> MSKPELKEDKMLEVHFVGDDDVLNHILDREGGAKLKKERAQLLVNPKKIIKKPEYDLEEDDQEVLKDQNYVEIMGRDVQESLKNGSATGGGNKVYSFQNRKHSEKMAKLASELAKTPQKSVSFSLKNDPEITINVPQSSKGHSASDKVQPKNNDKSEFLSTAPRSLRKRLIVPRSHSDSESEYSASNSEDDEGVAQEHEEDTNAVIFSQKIQAQNRVVSAPVGKETPSKRMKRDKTSDLVEEYFEAHSSSKVLTSDRTLQKLKRAKLDQQTLRNLLSKVSPSFSAELKQLNQQYEKLFHKWMLQLHLGFNIVLYGLGSKRDLLERFRTTMLQDSIHVVINGFFPGISVKSVLNSITEEVLDHMGTFRSILDQ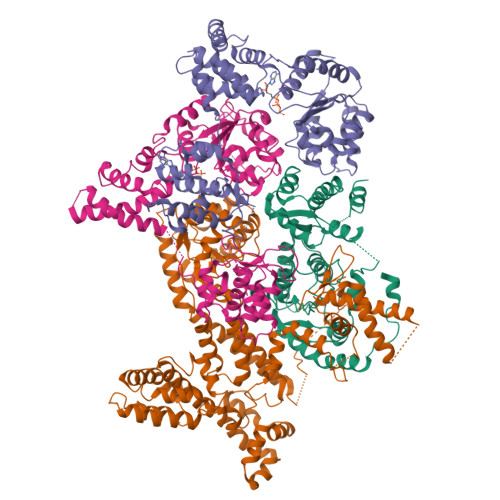LDWIVNKFKEDSSLELFLLIHNLDSQMLRGEKSQQIIGQLSSLHNIYLIASIDHLNAPLMWDHAKQSLFNWLWYETTTYSPYTEETSYENSLLVKQSGSLPLSSLTHVLRSLTPNARGIFRLLIKYQLDNQDNPSYIGLSFQDFYQQCREAFLVNSDLTLRAQLTEFRDHKLIRTKKGTDGVEYLLIPVDNGTLTDFLEKEEEEA;> MATSSMSKGCFVFKPNSKKRKISLPIEDYFNKGKNEPEDSKLRFETYQLIWQQMKSENERLQEELNKNLFDNLIEFLQKSHSGFQKNSRDLGGQIKLREIPTAALVLGVNVTDHDLTFGSLTEALQNNVTPYVVSLQAKDCPDMKHFLQKLISQLMDCCVDIKSKEEESVHVTQRKTHYSMDSLSSWYMTVTQKTDPKMLSKKRTTSSQWQSPPVVVILKDMESFATKVLQDFIIISSQHLHEFPLILIFGIATSPIIIHRLLPHAVSSLLCIELFQSLSCKEHLTTVLDKLLLTTQFPFKINEKVLQVLTNIFLYHDFSVQNFIKGLQLSLLEHFYSQPLSVLCCNLPEAKRRINFLSNNQCENIRRLPSFRRYVEKQASEKQVALLTNERYLKEETQLLLENLHVYHMNYFLVLRCLHKFTSSLPKYPLGRQIRELYCTCLEKNIWDSEEYASVLQLLRMLAKDELMTILEKCFKVFKSYCENHLGSTAKRIEEFLAQFQSLDETKEEEDASGSQPKGLQKTDLYHLQKSLLEMKELRRSKKQTKFEVLRENVVNFIDCLVREYLLPPETQPLHEVVYFSAAHALREHLNAAPRIALHTALNNPYYYLKNEALKSEEGCIPNIAPDICIAYKLHLECSRLINLVDWSEAFATVVTAAEKMDANSATSEEMNEIIHARFIRAVSELELLGFIKPTKQKTDHVARLTWGGC;> MSSRKSKSNSLIHTECLSQVQRILRERFCRQSPHSNLFGVQVQYKHLSELLKRTALHGESNSVLIIGPRGSGKTMLINHALKELMEIEEVSENVLQVHLNGLLQINDKIALKEITRQLNLENVVGDKVFGSFAENLSFLLEALKKGDRTSSCPVIFILDEFDLFAHHKNQTLLYNLFDISQSAQTPIAVIGLTCRLDILELLEKRVKSRFSHRQIHLMNSFGFPQYVKIFKEQLSLPAEFPDKVFAEKWNENVQYLSEDRSVQEVLQKHFNISKNLRSLHMLLMLALNRVTASHPFMTAVDLMEASQLCSMDSKANIVHGLSVLEICLIIAMKHLNDIYEEEPFNFQMVYNEFQKFVQRKAHSVYNFEKPVVMKAFEHLQQLELIKPMERTSGNSEREYQLMKLLLDNTQIMNALQKYPNCPTDVRQWATSSLSWL;> MPHLENVVLCRESQVSILQSLFGERHHFSFPSIFIYGHTASGKTYVTQTLLKTLELPHVFVNCVECFTLRLLLEQILNKLNHLSSSEDGCSTEITCETFNDFVRLFKQVTTAENLKDQTVYIVLDKAEYLRDMEANLLPGFLRLQELADRNVTVLFLSEIVWEKFRPNTGCFEPFVLYFPDYSIGNLQKILSHDHPPEYSADFYAAYINILLGVFYTVCRDLKELRHLAVLNFPKYCEPVVKGEASERDTRKLWRNIEPHLKKAMQTVYLREISSSQWEKLQKDDTDPGQLKGLSAHTHVELPYYSKFILIAAYLASYNPARTDKRFFLKHHGKIKKTNFLKKHEKTSNHLLGPKPFPLDRLLAILYSIVDSRVAPTANIFSQITSLVTLQLLTLVGHDDQLDGPKYKCTVSLDFIRAIARTVNFDIIKYLYDFL BUTYL-PHOSPHINIC ACID 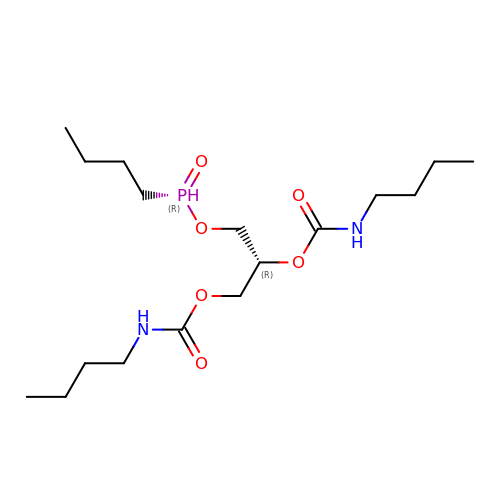2,3-BIS-BUTYLCARBAMOYLOXY-PROPYL ESTER GROUP | C17 H35 N2 O6 P | QWIXWBNJNKHHHW-OAHLLOKOSA-N>[3x]IAPTVWKLADRSKIYMADLESALHYILRIEVGRFPVLEGQRLVALKKFVAVLAKYFPGRPLVQNFLHSVNEWLKRQKRNKIPYSFFKTALDDRKEGAVLAKKV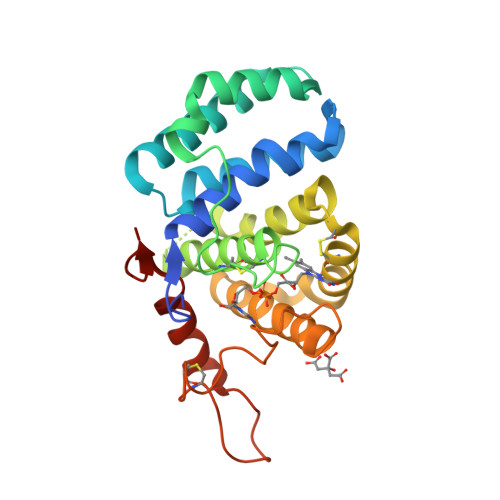NWIGCQGSEPHFRGFPCSLWVLFHFLTVQAARQNVDHSQEAAKAKEVLPAIRGYVHYFFGCRDCASHFEQMAAASMHRVGSPNAAVLWLWSSHNRVNARLAGAPSEDPQFPKVQWPPRELCSACHNERLDVPVWDVEATLNFLKAHFSPSNIILDFPA>[2x]MHHHHHHGSPLPATHDLHISGSINGHE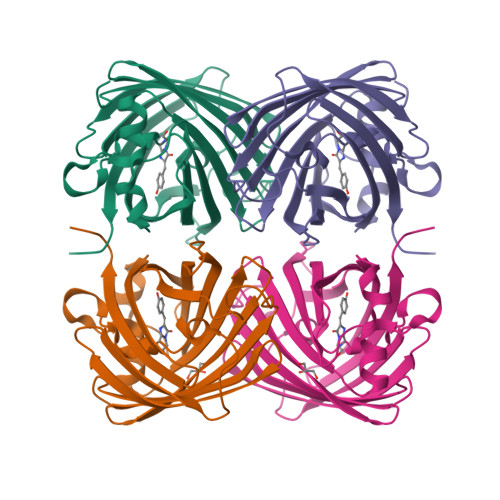FDLEGSGKGNAKEGYQELHLKSNKGDLSFSPWILVPNIGYGFYQYLPFPDGAMSPYQAAMHDGSGYVMHRSMQFEDGAMLHSDHRYIYKGNHIKGEFRLTGSGFPADGPVMTNSLTAADWCVDKLLYPNDNTIIGKFDWTYTTTSGKRYQSDVQTNVTFGKPIAADILKKQPMFVFRKVELKHTKTELNFKQWQKAFQDIA3-((4-(6-chloro-2-(1,3-dimethyl-1H-pyrazol-4-yl)-3H-imidazo[4,5-b]pyridin-7-yl)-1H-pyrazol-1-yl)methyl)-5-methylisoxazole 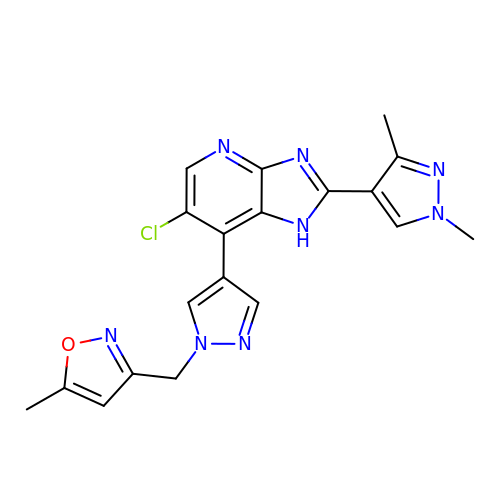| C19 H17 Cl N8 O | FZRLFVHIDOFKIN-UHFFFAOYSA-N(4Z)-6-bromo-4-({[4-(pyrrolidin-1-ylmethyl)phenyl]amino}methylidene)isoquinoline-1,3(2H,4H)-dione | C21 H20 Br 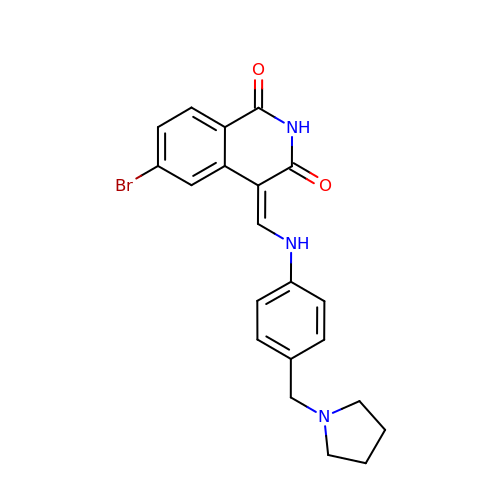N3 O2 | JFEKAVPMVOLVTH-UNOMPAQXSA-N> SSHEQFRAALQLVVDPGDPRSYLDNFIKIGEGSTGIVCIATVRSSGKLVAVKKM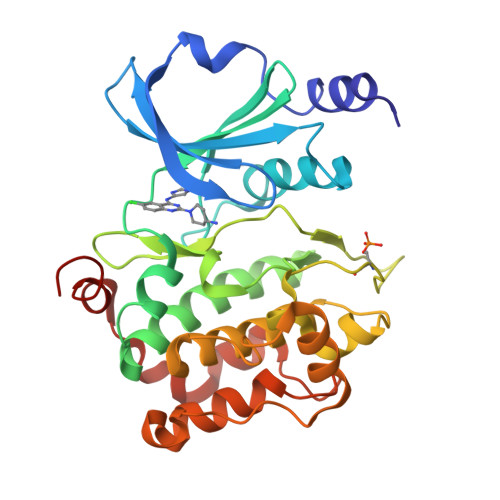DLRKQQRRELLFNEVVIMRDYQHENVVEMYNSYLVGDELWVVMEFLEGGALTDIVTHTRMNEEQIAAVCLAVLQALSVLHAQGVIHRDIKSDSILLTHDGRVKLSDFGFCAQVSKEVPRRKSLVGTPYWMAPELISRLPYGPEVDIWSLGIMVIEMVDGEPPYFNEPPLKAMKMIRDNLPPRLKNLHKVSPSLKGFLDRLLVRDPAQRATAAELLKHPFLAKAGPPASIVPLMRQN Mycobacterium tuberculosis DNA gyrase, an indispensable nanomachine involved in the regulation of DNA topology, is the only type II topoisomerase present in this organism and is hence the sole target for quinolone action, a crucial drug active against multidrug-resistant tuberculosis. DNA gyrase and topoisomerase IV consist of two subunits (GyrA and GyrB in DNA gyrase, ParC and ParE in topoisomerase IV), which form the catalytically active heterotetrameric complex (i.e. A2B2 and C2E2, respectively). The GyrB Toprim and GyrA breakage-reunion domains come from separate subunits and cooperatively form the enzyme core. The breakage-reunion domain contains the catalytic tyrosine responsible for the cleavage and religation of the DNA double helix.

The crystal structure of the breakage-reunion domain we solved to 2.7 Å resolution, revealed a promising interaction that will be further exploited for drug design. This interaction involves the N-terminal helix, which is anchored in the active site of a symmetry-related molecule. The crystals belong to space group C2, with a dimer in the asymmetric unit. Consequently, the final model spans residues 9 to 499 for chain A and 29 to 501 for chain B. GA57BK forms a biological dimer in a ‘closed’ conformation in the asymmetric unit, as the C-gate, which constitutes the so-called primary dimer interface, and the DNA-gate, the secondary protein-protein interface, are both closed. In contrast to other structures of the breakage-reunion domain alone (i.e. E. coli DNA gyrase, S. aureus and S. pneumoniae topoisomerase IV), the N-terminal segment of GA57BK (residues 9–41) is ordered and is organized in two distinct secondary structures. Residues D9 to E16 form a loop whose B factors indicate high flexibility, followed by a 24-residue long α-helix. The α-helix is deeply anchored in the active site of its neighbouring molecule. In addition, D30 establishes hydrogen bonds with the hydroxyl group of the catalytic tyrosine (Y129) and a salt bridge with the catalytic arginine (R128). The presence of this N-terminal helix would prevent DNA binding.

>MTDTTLPPDDSLDRIEPVDIEQEMQRSYIDYAMSVIVGRALPEVRDGLKPVHRRVLYAMFDSGFRPDRSHAKSARSVAETMGNYHPHGDASIYDSLVRMAQPWSLRYPLVDGQGNFGSPGNDPPAAMRYTEARLTPLAMEMLREIDEETVDFIPNYDGRVQEPTVLPSRFPNLLANGSGGIAVGMATNIPPHNLRELADAVFWALENHDADEEETLAAVMGRVKGPDFPTAGLIVGSQGTADAYKTGRGSIRMRGVVEVEEDSRGRTSLVITELPYQVNHDNFITSIAEQVRDGKLAGISNIEDQSSDRVGLRIVIEIKRDAVAKVVINNLYKHTQLQTSFGANMLAIVDGVPRTLRLDQLIRYYVDHQLDVIVRRTTYRLRKANERAHILRGLVKALDALDEVIALIRASETVDIARAGLIELLDIDEIQAQAILDMQLRRLAALERQRIIDDLAKIEAEIADLEDILAKPERQRGIVRDELAEIVDRHGDDRRTRIIAAEHHHHHH[2x]> VDLSNLPRVKHTLVPPPFAHAHEQVAASGPVINEFEMRIIEKEVQLDEDAYLQAMTFDGSIPGPLMIVHEGDYVELTLINPPENTMPHNIDFHAATGALGGGGLTLINPGEKVVLRFKATRAGAFVYHCAPGGPMIPWHVVSGMAGCIMVLPRDGLKDHEGKPVRYDTVYYIGESDHYIPKDEDGTYMRFSDPSEGYEDMVAVMDTLIPSHIVFNGAVGALTGEGALKAKVGDNVLFVHSQPNRDS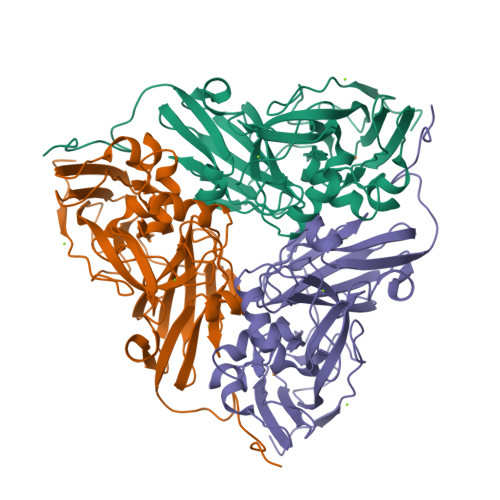RPHLIGGHGDLVWETGKFHNAPERDLETWFIRGGTAGAALYKFLQPGVYAYVNHNLIEAVHKGATAHVLVEGEWDNDLMEQVVAPVG> MGSDKIHHHHHHMGIDELYKKEFGIVAGVDEAGRGCLAGPVVAAAVVLEKEIEGINDSKQLSPAKRERLLDEIMEKAAVGIGIASPEEIDLYNIFNATKLAMNRALENLSVKPSFVLVDGKGIELSVPGTCLVKGDQKSKLIGAASIVAKVFRDRLMSEFHRMYPQFSFHKHKGY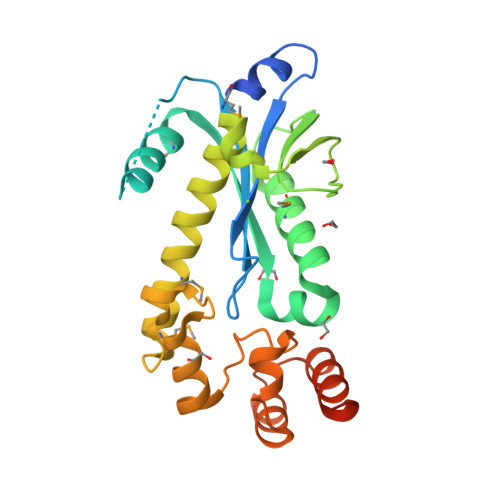ATKEHLNEIRKNGVLPIHRLSFEPVLELLTDDLLREFFEKGLISENRFERILNLLGARKSVVFRKERTNHNLPLF>[2x]KSCPNPGEIRNGQIDVPGGILFGATISFSCNTGYKLFGSTSSFCLISGSSVQWSDPLPECREIYCPAPPQIDNGI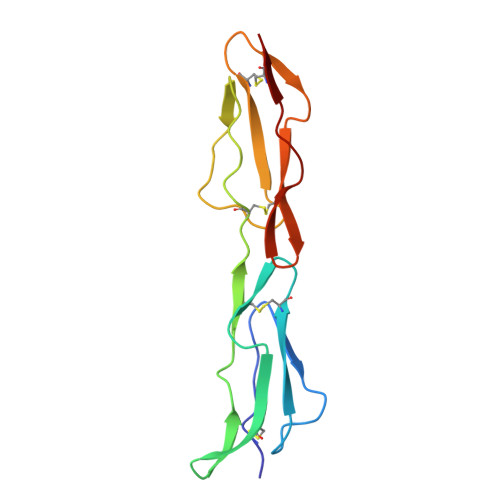IQGERDHYGYRQSVTYACNKGFTMIGEHSIYCTVNNDEGEWSGPPPECRG> GTFTGIDPFTGTQACITAASAVSGIIADLDTTIMFATAGTLNREGAETFADHREGILKTAKVLVEDTKVLVQNAAGS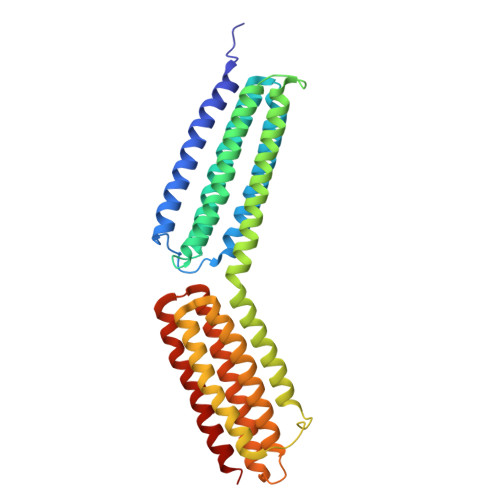QEKLAQAAQSSVATITRLADVVKLGAASLGAEDPETQVVLINAVKDVAKALGDLISATKAAAGKVGDDPAVWQLKNSAKVMVTNVTSLLKTVKAVEDEATKGTRALEATTEHIRQELAVFCSPEPPAKTSTPEDFIRMTKGITMATAKAVAAGNSCRQEDVIATANLSRRAIADMLRACKEAAFHPEVAPDVRLRALHYGRECANGYLELLDHVLLTLQKPNPDLKQQLTGHSKRVAGSVTELIQAAEAMKGT>[7x]GAGALSPKAATLAERSAGLAFSLYQAMAKDQAVENILLSPVVVASSLGLVSLGGKATTASQAKAVLSAEQLRDEEVHAGLGELLRSLSNSTARNVTWKLGSRLYGPSSVSFAEDFVRSSKQHYNCEHSKINFRDKRSALQSINEWAAQ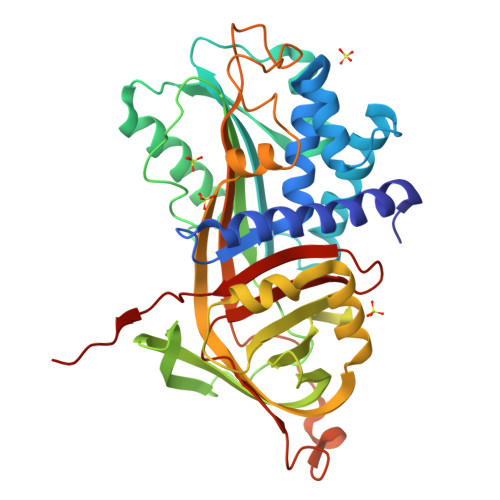TTDGKLPEVTKDVERTDGALLVNAMFFKPHWDEKFHHKMVDNRGFMVTRSYTVGVTMMHRTGLYNYYDDEKEKLQIVEMPLAHKLSSLIILMPHHVEPLERLEKLLTKEQLKIWMGKMQKKAVAISLPKGVVEVTHDLQKHLAGLGLTEAIDKNKADLSRMSGKKDLYLASVFHATAFEWDTEGNPFDQDIYGREELRSPKLFYADHPFIFLVRDTQSGSLLFIGRLVRPKGDKMRDEL> MASSSTPRFRVYSKYLFLTYPQCTLEPQYALDSLRTLLNKYEPLYIAAVRELHEDGSPHLHVLVQNKLRASITNPNALNLRMDTSPFSIFHPNIQAAKDCNQVR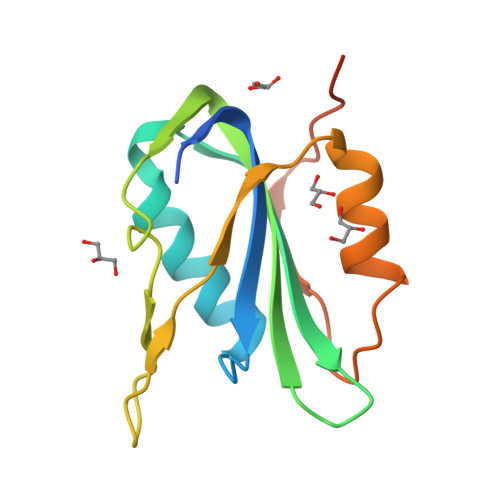DYITKEVDSDVNTAEWGTFVAVSTPGRKDRDAD>MEKKMSGSRPTQSSEGSRRSRHSARIIAQTTVDAKLHADFEESGSSFDYSTSVRVTGPVVENQPPRSDKVTTTYLHHIQKGKLIQPFGCLLALDEKTFKVIAYSENASELLTMASHAVPSVGEHPVLGIGTDIRSLFTAPSASALQKALGFGDVSLLNPILVHCRTSAKPFYAIIHRVTGSIIIDFEPVKPYEVPMTAAGALQSYKLAAKAITRLQSLPSGSMERLCDTMVQEVFELTGYDRVMAYKFHEDDHGEVVSEVTKPGLEPYLGLHYPATDIPQAARFLFMKNKVRMIVDCNAKHARVLQDEKLSFDLTLCGSTLRAPHSCHLQYMANMDSIASLVMAVVVNEEDGEGDAPDATTQPQKRKRLWGLVVCHNTTPRFVPFPLRYACEFLAQVFAIHVNKEVELDNQMVEKNILRTQTLLCDMLMRDAPLGIVSQSPNIMDLVKCDGAALLYKDKIWKLGTTPSEFHLQEIASWLCEYHMDSTGLSTDSLHDAGFPRALSLGDSVCGMAAVRISSKDMIFWFRSHTAGEVRWGGAKHDPDDRDDARRMHPRSSFKAFLEVVKTRSLPWKDYEMDAIHSLQLILRNAFKDSETTDVNTKVIYSKLNDLKIDGIQELEAVTSEMVRLIETATVPILAVDSDGLVNGWNTKIAELTGLSVDEAIGKHFLTLVEDSSVEIVKRMLENALEGTEEQNVQFEIKTHLSRADAGPISLVVNACASRDLHENVVGVCFVAHDLTGQKTVMDKFTRIEGDYKAIIQNPNPLIPPIFGTDEFGWCTEWNPAMSKLTGLKREEVIDKMLLGEVFGTQKSCCRLKNQEAFVNLGIVLNNAVTSQDPEKVSFAFFTRGGKYVECLLCVSKKLDREGVVTGVFCFLQLASHELQQALHVQRLAERTAVKRLKALAYIKRQIRNPLSGIMFTRKMIEGTELGPEQRRILQTSALCQKQLSKILDDSDLESIIEGCLDLEMKEFTLNEVLTASTSQVMMKSNGKSVRITNETGEEVMSDTLYGDSIRLQQVLADFMLMAVNFTPSGGQLTVSASLRKDQLGRSVHLANLEIRLTHTGAGIPEFLLNQMFGTEEDVSEEGLSLMVSRKLVKLMNGDVQYLRQAGKSSFIITAELAAANK[2x]

Phytochromes (phys), first discovered in plants, are red and far-red photoreceptors that are also widely found in bacteria and fungi later. PhyA is distinct from other phys and is responsible for the very low fluence response (VLFR) under a broad spectrum of light and for the far-red light high irradiance response (FR-HIR). In higher plants, phys share a conserved domain structure consisting of an N-terminal photosensory module (PSM) followed by two tandem Period/ARNT/Singleminded (PAS) domains, and a C-terminal histidine kinase-related domain (HKRD). Then, we solved cryo-electron microscopy (cryo-EM) structures of apo-AtphyA, AtphyA-Pr and ZmphyA1-Pr at resolutions of 3.8 Å, 3.0 Å and 3.3 Å, respectively.

Structural comparison of apo-AtphyA and AtphyA-Pr revealed that they share a highly similar homodimeric structure. However, notable differences were found around the PΦB-binding cradle. Except for those in the GAF helix-α5, the key residues involved in PΦB binding retain similar conformations in apo and Pr states of phyA. Tyr327 of apo-phyA helix-α5 can cause obvious steric clash with the D ring of PΦB. Thus, helix-α5 of AtphyA-Pr moves outwards, to accommodate the bulk of PΦB and facilitate the formation of covalent thioether linkage between them. Similarly, in AtphyA-Pr, the PRSSF motif contacts GAF helix-α5 through hydrophobic interaction with its Phe554. Nonetheless, this contact is probably abolished in apo-AtphyA, as a closer location of GAF helix-α5 might cause substantial steric clashes with the PRSSF motif. Thus, the portion downstream of the WGG motif in the PHY tongue of apo-phyA becomes more disordered than that of phyA-Pr, facilitating the entrance of PΦB to its pocket. Size-exclusion chromatography assays demonstrated that PΦB-free phyA (apo-phyA) and Pr conformer of phyA (phyA-Pr) have a similar molecular weight of ~250 kDa.>[2x]AIINLLRELEIYGMQYANSHQYTYGSSYSDDTNPIRIAGLDARIPDPIVTDPVNHIVLDRRIITN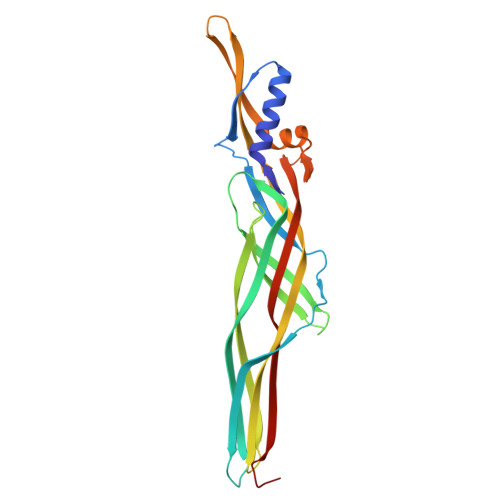TTSNSLEGVFSFSNAYTSRTSSQTRDGVTAGTNITGKYFANLFFEQVGLSGRIAFEGAVTNENKYTLDATQDFRDSQTIRVPPFHRATGVYTLEQGAFEKMTVLECVVSGNGIIRYYRTLPDNSYTEIVQRVNIIDVLQANGTPGFTISKEQNRAYFTGEGTISGQIGLQTFIDVVIEPLPGHA(2~{S})-1-methoxypropan-2-amine | C4 H11 N O | 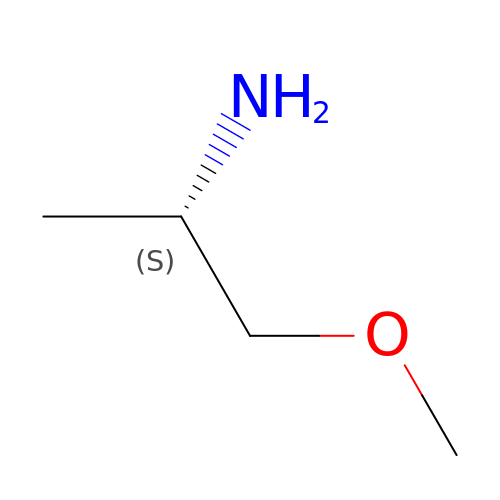NXMXETCTWNXSFG-BYPYZUCNSA-N> GSMEGAGAGSGFRKELVSRLLHLHFKDDKTKVSGDAL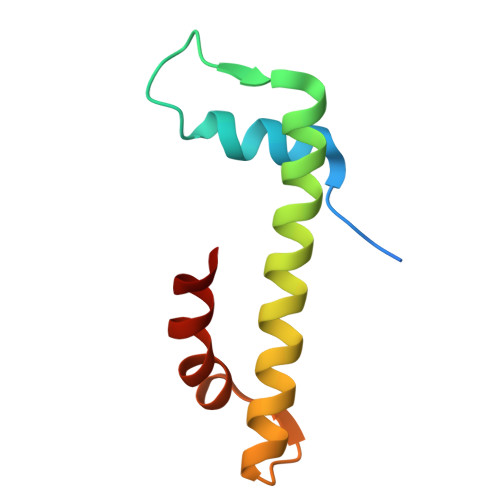QLMVELLKVFVVEAAVRGVRQAQAEDALRVDVDQLEKVLPQLLLDF NrdR, an RNR-specific repressor, controls the transcription of RNR genes and, often, its own, in most bacteria and some archaea. NrdR senses the concentration of nucleotides through its ATP-cone, an evolutionarily mobile domain that also regulates the enzymatic activity of many RNRs, while a Zn-ribbon domain mediates binding to NrdR boxes upstream of and overlapping the transcription start site of RNR genes. NrdRs (140–220 residues) consist of an N-terminal Zn-ribbon domain followed by an ATP-cone domain and in some cases a C-terminal part of variable length and unknown function. In contrast to all earlier suggested mechanisms, we show that the NrdR monomer contains two nucleotide-binding sites, one inner site that binds ATP and one more exposed site that can bind either ATP or dATP.

The structure of dATP/ATP-loaded NrdR in the absence of DNA (3.1 Å resolution) reveals an octameric complex composed of two tetrameric assemblies. 2D classification of this dataset showed a particle population consisting predominantly of NrdR octamers, with a small population of NrdR tetramers. Apart from a slight adjustment of the angles of the Zn-ribbon domains the two tetramers in the octamer are virtually identical to the tetramer that interacts with DNA. Tetramers competent to bind DNA are locked in an octameric form in which the Zn-ribbons of two tetramers face each other. The octamer would therefore need to dissociate to bind DNA. PISA analysis reveals that ~3700 Å2 of SAA are buried in four distinct small interaction areas between tetramers, compared to ~8550 Å2 buried within each tetramer. This implies that interactions between tetramers are significantly weaker than those within tetramers. The predicted free energy of dissociation of about –13 kcal/mol suggests that the octamer is unstable or marginally stable in solution, thus liable to dissociate into tetramers. This oligomerization mechanism may provide an additional layer of regulation by controlling the concentration of tetrameric NrdR, available for binding the promoters. In the octamer, the 6-NH2 group of dATP makes an H-bond to the main-chain carbonyl group of a neighboring monomer.

>[8x]MHCPFCRHPDSRVVDSRTTDDGTSIRRRRQCPDCSRRFTTVETCSLMVVKRSGVTEPFSRTKVINGVRKACQGRPVTEDALAQLGQRVEEAVRATGSAELTTHDVGLAILGPLQELDLVAYLRFASVYRAFDSLEDFEAAIAELRETTGHPGEEDDTGAGSQENDRGPTGAGQVPEPAGAADKLAAALEHHHHHH> GPLGSPEFMINGVSLQGTAGYEAHTEEGNVNVKKLLESLNSKSLGDMDKDSELAATLQKMINPSGGDGNSSGCALHACMAMLGYGVREAPVPNEISEYMTGFFHRHLEQIDSEGIVSHPNETYSKFRERIAENILQNTSKGSVVMISIEQATHWIAGFNDGEKIMFLDVQTGKGFNLYDPVEKSPDAFVDENSSVQVIHVSDQEF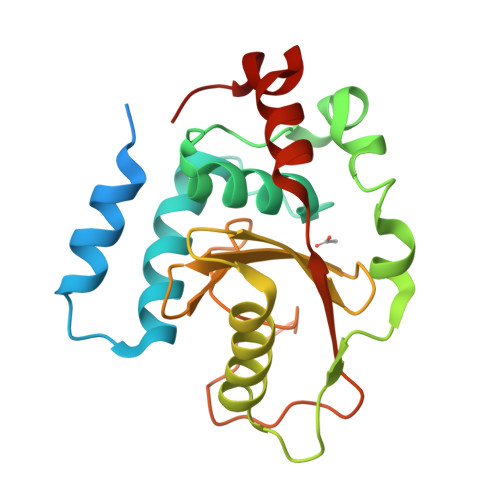DHYANSSSWKSKRLC>MASHERTQPQNMAFRAKATRTARRESQETFWSRFGISQS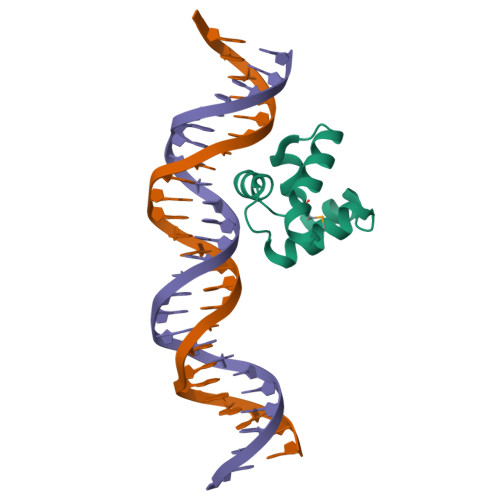CGSRFENGENLPFPIYLLLHFYIEGQITDRQLADLRGKIRE[2x]>[2x]MQNVGFIGWRGMVGSVLMQRMVEERDFDAIRPVFFSTSQLGQAAPSFGGTTGTLQDAFDLEALKALDIIVTCQGGDYTNEIYPKLRESGWQGYWIDAASSLRMKDDAIIILDPVNQDVITDGLNNGIRTFVGGNCTVSLMLMSLGGLFANDLVDWVSVATYQAASGGGARHMRELLTQMGHLYGHVADELATP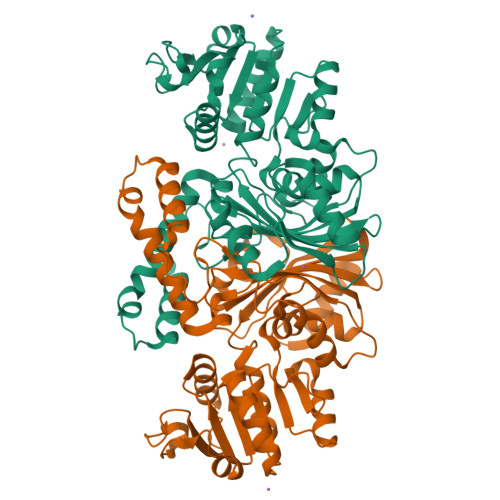SSAILDIERKVTTLTRSGELPVDNFGVPLAGSLIPWIDKQLDNGQSREEWKGQAETNKILNTSSVIPVDGLCVRVGALRCHSQAFTIKLKKDVSIPTVEELLAAHNPWAKVVPNDREITMRELTPAAVTGTLTTPVGRLRKLNMGPEFLSAFTVGDQLLWGAAEPLRRMLRQLA> MRMDEFYTKVYDAVCEIPYGKVSTYGEIARYVGMPSYARQVGQAMKHLHPETHVPWHRVINSRGTISKRDISAGEQRQKDRLEEEGVEIYQTSLG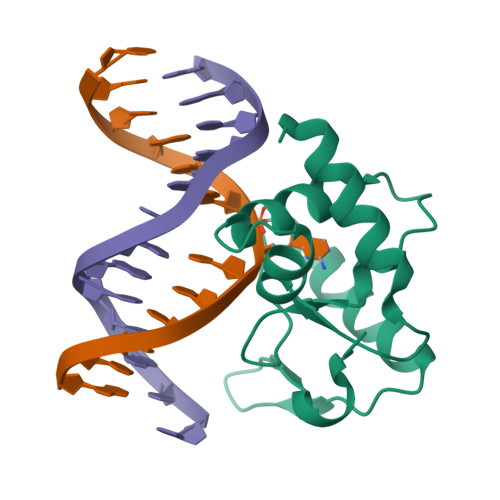EYKLNLPEYMWKPGSHHHHHH>SYSIEVRTHSALHVVKGAVVKTAGSDAKWTTSTYVKGNKGVLIVKAALEPDKWGIAAIEALANEKVKENAPIKIYELPREEAEKMFGEDMYDLFPVPEDVRILKVVVIEDWNVNACNKEHTKTTGEIGPIKIRKVRFR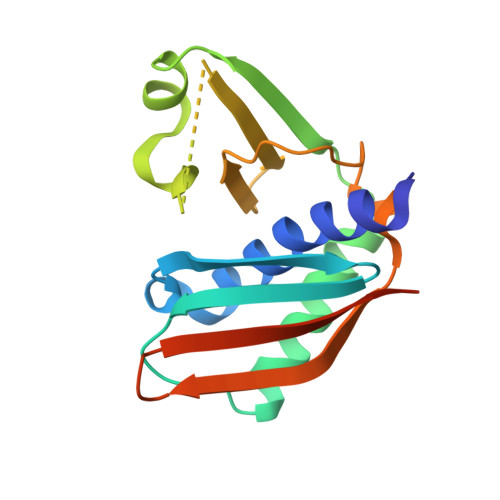KSKGLLEIHFELLELEHHHHHH[2x]Adenosine undergoes ATP-dependent phosphorylation catalyzed by adenosine kinase (ADK). In plants, ADK also phosphorylates cytokinin ribosides, transport forms of the hormone. We discovered that maize and moss enzymes can form dimers upon increasing protein concentration, setting them apart from the monomeric human and protozoal ADKs. Structural and kinetic analyses revealed a catalytically inactive unique dimer.

The asymmetric unit contains one monomer for the ZmADK3–AP5A complex and two monomers for the PpADK1–Ado–ADP complex, all in the closed conformation. Structural comparison between ZmADK2 (open state) and the closed state of both ZmADK3 and PpADK1 reveals that AP5A (or Ado) binding induced a rigid-body motion of the smaller domain towards the large domain, resulting in the closed conformation. Two helices, α1 and α2, shift by up to 12 Å to shield the Ado site from the solvent. The electron density map of the bisubstrate analog AP5A in ZmADK3 is very well defined. The ligand binds in the groove between the large and small domains. The purine ring of Ado stacks on the phenyl ring of Phe169 (in ZmADK3 numbering; PpADK1 numbering is shifted lower by three amino acids) and establishes hydrophobic interactions with Leu17, Ala66, Cys123, Leu134, and Ala136. The N1 and N3 atoms of the purine ring are H-bonded to the side chain of Asn15 and the main chain nitrogen atom of Ala66, respectively. Both O2' and O3' atoms of the ribose moiety bind to the side chain of Asp19. The γ-phosphate in AP5A forms a hydrogen bond with the OG1 atom of Thr294 and the side chain of Arg132. AP5A in ZmADK3 and AMP-PCP in ZmADK2 adopt the same conformation and position in the ATP-binding site. To form the closed ternary complex and bring the two subunits close together, the enzyme must be monomeric as shown by the structures of both ZmADK3 bound to AP5A and PpADK1 bound to ADP and Ado.

> MGSSHHHHHHSQDPNSSSASSGYEGILLGMGNPLLDISAVVDEGFLAKYDVKPGNAILAEDKHLPMYDELASKSNVEYIAGGATQNSIRVAQWMLQIPGASSYIGCIGKDKFGEEMKKNAQAAGINAHYHEDENAPTGTCAVCVVGGERSLIANLSAANCYKSEHLKKPENWALVEKAKYIYIAGFFLTVSPDSIQLVAEHAAATNKVFMMNLSAPFICEVFRDAQEKALPYVDYIFGNETEARTFAKVRGWETENVEEIALKISQLPKASGTHKKITVITQGCDPVVVADDGKVKTFPVILLPKEKLVDTNGAGDAFVGGFLSQLVQEKNIDECVRAACYAANVVIQRSGCTYPEKPDFN>MAASQEIFLQVLNLADGDVKVTVLGSRNNSLLVESVSSFQNTTHYSKLH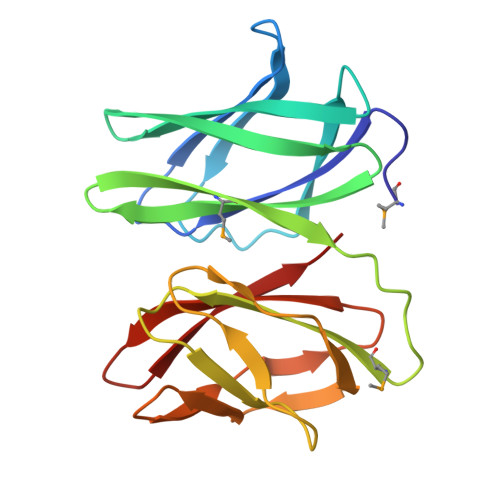LEAKSQDLHFHLKYNSLSVHNDHSVEEKNCYQLLIHQDGESISSMLVKDTGIKPANGMAAIRFINTLHKDLNISLDTDAPLSVGKDYGVSAYRTVLRGKYPAVHCETEDKVFSLDLGQLDFGTTYLFVITNITSQGLQAWKAEDI[3x]> MARRILVVEDEAPIREMVCFVLEQNGFQPVEAEDYDSAVNQLNEPWPDLILLAWMLPGGSGIQFIKHLRRESMTRDIPVVMLTARGEEEDRVRGLETGADDCITKPFSPKELVARIKAVMRRISPMA;> MARRILVVED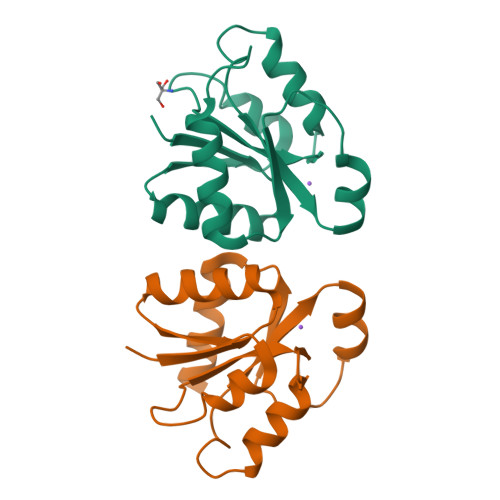EAPIREMVCFVLEQNGFQPVEAEDYDSAVNQLNEPWPDLILLAWMLPGGSGIQFIKHLKRESMTRDIPVVMLTARGEEEDRVRGLETGADDCITKPFSPKELVARIKAVMRRISPMA> DAPGQYGAYFHDDGFLAFPGHVFSRSLPEVPETIELEVRTSTASGLLLWQGVEVGEAGQGKDFISL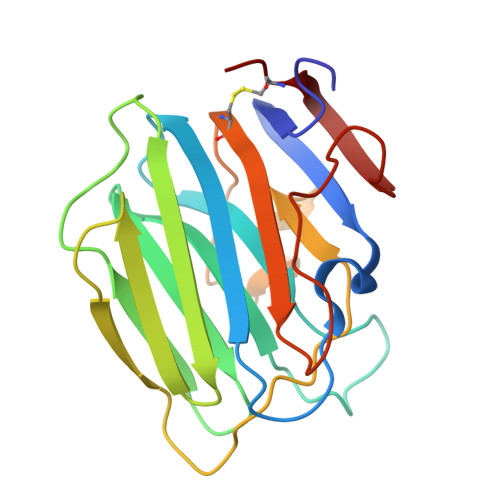GLQDGHLVFRYQLGSGEARLVSEDPINDGEWHRVTALREGRRGSIQVDGEELVSGRSPGPNVAVNAKGSVYIGGAPDVATLTGGRFSSGITGCVKNLVLHSARPGAPPPQPLDLQHRAQAGANTRPCPS>[4x]MNLEDLKLLKEAVMFTAEDEEYIQKAGEVLEDQVEEILDTWYGFVGSHPHLLYYFTSPDGTPNEKYLAAVRKRFSRWILDTSNRSYDQAWLDYQYEIGLRHHRTKKNQTDNVESVPNIGYR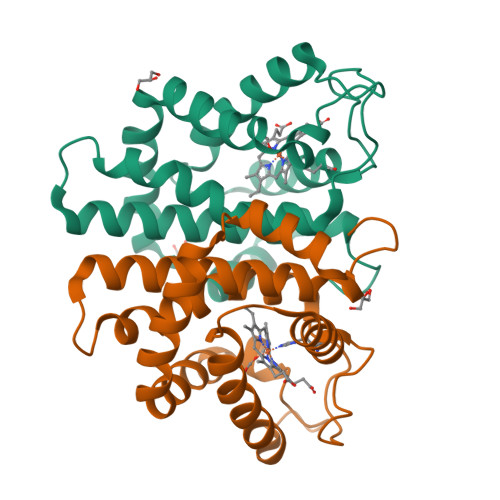YLVAFIYPITATMKPFLARKGHTPEEVEKMYQAWFKATTLQVALWSYPYVKYGDF>KSPSAQELKEQGNRLFVGRKYPEAAACYGRAITRNPLVAVYYTNRALCYLKMQQHEQALADCRRALELDGQSVKAHFFLGQCQLEMESYDEAIANLQRAYSLAKEQRLNFGDDIPSALRIAKKKRWNS[2x];>XSIDM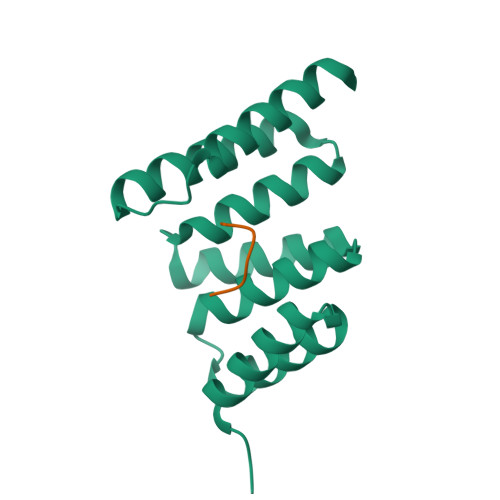VD[2x]>ASMTGGQQMGRGSEFMGQ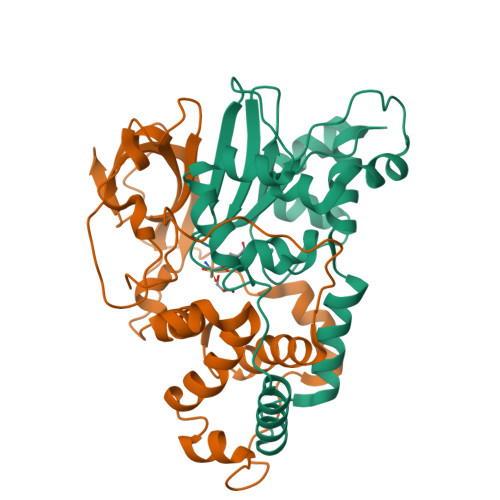SHTHDHHHDGYQAPPEDIALRVKALESLLIEKGLVDPAAMDLVVQTYEHKVGPRNGAKVVAKAWVDPAYKARLLADGTAGIAELGFSGVQGEDMVILENTPAVHNVFVCTLCSCYPWPTLGLPPAWYKAAPYRSRMVSDPRGVLAEFGLVIPANKEIRVWDTTAELRYMVLPERPAGTEAYSEEQLAELVTRDSMIGTGLPTQPTPSH[4x];>MNGIHDTGGAHGYGPVYREPNEPVFRYDWEKTVMSLLPALLANGNFNLDEFRHSIERMGPAHYLEGTYYEHWLHVFENLLVEKGVLTATEVATGKAASGKTATPVLTPAIVDGLLSTGASAAREEGARARFAVGDKVRVLNKNPVGHTRMPRYTRGKVGTVVIDHGVFVTPDTAAHGKGEHPQHVYTVSFTSVELWGQDASSPKDTIRVDLWDDFLEPA[4x]> MIRNVKKQRPVNLDLQTI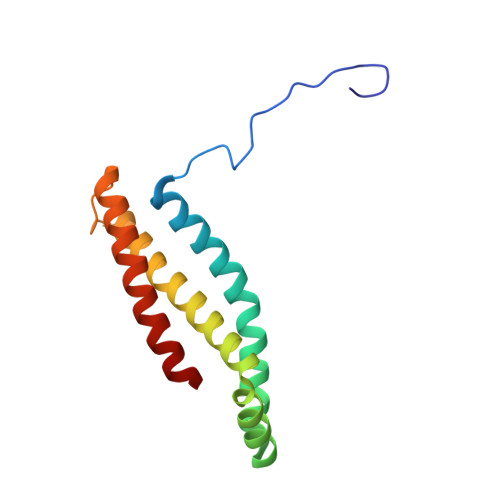RFPITAIASILHRVSGVITFVAVGILLWLLGTSLSSPEGFEQASAIMGSFFVKFIMWGILTALAYHVVVGIRHMMMDFGYLEETFEAGKRSAKISFVITVVLSLLAGVLVW SulE, an esterase, which detoxifies a variety of sulfonylurea herbicides through de-esterification, provides an attractive approach to remove environmental sulfonylurea herbicides and develop herbicide-tolerant crops. SulE catalyzes the de-esterification of a variety of sulfonylurea herbicides, such as MM, BM, SM, TM, TrM, EM, and CE, to the corresponding herbicidal-inactive parent acid. The structures show that SulE is a dimer with a lid loop in a domain-swapped β-hairpin covering the active site from the opposing monomer. SulE shows a similar catalytic triad consisting of Ser209, His333, and Glu232 at its active site.

To elucidate the catalytic mechanism of SulE, we solved the crystal structures of wild-type SulE in complex with CA, mutant S209A in complex with MM, and mutant S209A/H333A in complex with MM, SM, TM, TrM, EM, BM, and CE in the range of 1.29–1.63 Å. In the other six substrate-bound complex structures of S209A/H333A, clear electron density also could be observed for SM, AM, CE, and TrM, but the density for BM and TM were relatively poor. However, in the S209A/H333A-TM complex structure, Gly78 and Ala210 form hydrogen bonds with the oxygen atom of the sulfonyl group, while the ester O atom forms a hydrogen bond with the water molecule Wat801. In addition, superimposition of the structures of apo-SulE and S209A/H333A-TM complex showed that the oxymethyl group of TM and the imidazole ring of H333 side chain are incompatible with each other, indicating that the ester bond of TM is bound in an invalid position at the active site of the mutant S209A/H333A. Superposition of S209A/H333A-TM and P44R/S209A/H333A-TM complexes revealed no significant structural differences, and also no conformational changes occurred in TM. Different from the binding of TM in the active site of S209A/H333A, the ester bond of TM is located at a correct position, ready for catalysis in the active site of P44R/S209A/H333A. However, the electron density of TM is unclear, especially the sulfonylurea bridge and heterocyclic moiety, and the overall electron density is worse than that observed in the S209A/H333A active site, indicating that TM was bound more unstable in P44R/S209A/H333A than in S209A/H333A.

>[2x]METDNVELAQSKRKVVLAEQGSFYIGGRTVTGPGKFDPSKPVIRYSNEGATFYINQMYVNFQAPVRPRGLPLVFWHGGGLTGHIWESTPDGRPGFQTLFVQDRHTVYTIDQPGRGRGNIPTFNGPFGQLEEESIVNTVTGNSSKEGAWVRDRLGPAPGQFFENSQFPRGYEDNYFKEMGFSPSISSDEIVDAVVKLVTHIGPCVLVTHAASGVLGMRVATHAKNVRGIVAYEPATSIFPKGKVPEIPPLADKKSQIFPPFEIQESYFKKLAKIPIQFVFGDNIPKNPKSAYWFLDWWRVTRYAHSLSLEAINKLGGQASLLDLPTAGLRGNTAFPFTDRNNVQVASLLSDFLGKHGLDQNESLEHHHHHH>DLADRFAELERRYDARLGVYVPATGTTAAIEYRADERFAFCSTFKAPLVAAVLHQNPLTHLDKLITYTSDDIRGISPVAQQHVQTGMTIGQLCDAAIRYSDGTAANLLLADLGGPGGGTAAFTGYLRSLGDTVSRLDAEEPELNRDPPGDERDTTTPRAIALVLQQLVLGNALPPDKRALLTDWMARNTTGAKRIRAGFPADWKVIDKTGTGGYGRANDIAVVWSPTGVPYVVAVMSDRAGGGYDAEPREALLAEAATCVAGVLA[2x]

BlaC is a class A serine β‐lactamase found in Mycobacterium tuberculosis (Wang et al., 2006). The enzymes in this class utilize an active site serine (Ser70) to perform a nucleophilic attack on β‐lactam rings, forming a covalent acyl‐enzyme intermediate that is subsequently hydrolyzed (Fisher & Mobashery, 2009; Strynadka et al., 1992). BlaC can efficiently hydrolyze penicillin antibiotics but has low activity against later‐generation oxyimino‐cephalosporins, such as ceftazidime, due to their bulky C7β aminothiazole‐oxyimino side chain (Sun et al., 2023; Wang et al., 2006). We analyzed the structural changes in mutants of the β‐lactamase BlaC from Mycobacterium tuberculosis obtained via directed evolution for increased ceftazidime hydrolysis activity.

At 37°C, two variants were found that were further evolved, yielding P167S/D240G/D172A/S104G/H184R (PDDSH) and P167S/D240G/I105F/H184R (PDIH) in G3, respectively. The crystal structures of BlaC variants PD, PDDS, and PDDSH were solved at 1.3, 1.6, and 1.4 Å resolution, respectively. While the refinement statistics for the PD and PDDS structures are within the expected values for the resolution (Rfree of 18 and 17, respectively), the PDDSH dataset suffers from translational non‐crystallographic symmetry, resulting in a higher Rfree value of 25. As a consequence, the chain between residues 167 and 172 is only partially ordered, indicating mobility in this region of the Ω‐loop. In the BlaC variant PDDSH (purple in Figure 3a), the Ω‐loop residues 165–172 are disordered, indicating still more conformational flexibility. In this variant, the peptide bond between Gly104 and Ile105 is flipped, and the gatekeeper loop moves 2.5 Å compared to the PD and PDDS variants, enlarging the active site. Mutation H184R occurred twice, in different branches of the directed evolution experiments and in both cases causes an increase in the melting temperature, suggesting, therefore, that this mutation is generally stabilizing. An Arg at position 184 could potentially form salt bridges with Glu59 and Asp63 and a cation‐π interaction with Tyr48. The mutants selected at 37°C display more than 15‐fold increased resistance compared to PD and over 120‐fold compared to WT. For one branch of the directed evolution experiment, we managed to obtain crystal structures of the successive mutants, PD, PDDS, and PDDSH, showing the opening and increasing disorder of the Ω‐loop in an otherwise defined protein structure, suggesting minor structural changes.> KERAHQKRSSKRAPQMDW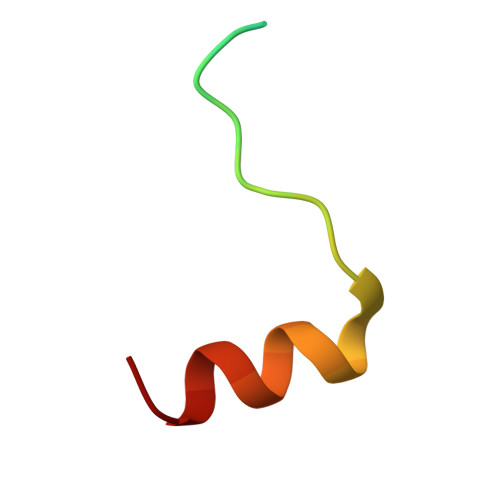SKKNELFSNL N-[5-[(4-BROMOPHENYL)METHYL]-4-HYDROXY-1,3-THIAZOL-2-YL]NAPHTHALENE-1-SULFONAMIDE | C20 H15 Br N2 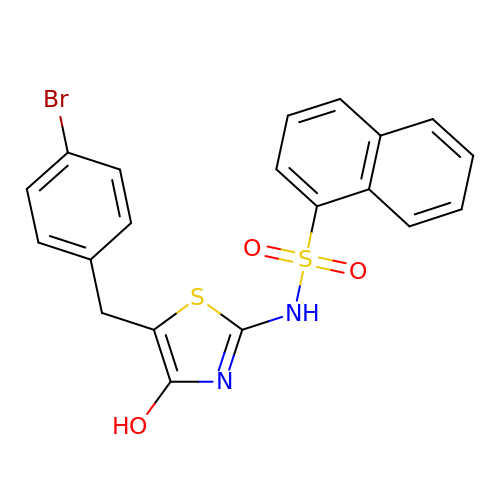O3 S2 | ULFLIVGUMGQSSF-UHFFFAOYSA-N>MHHHHHHSNKKSLSVIFVKPPFQLKKKFQKDPFYEI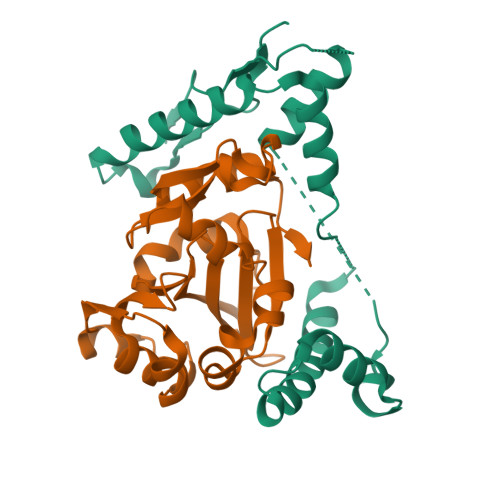EMRKQLQMQQDGINNMTIFEWLKNRENFKKYGRNPKSKKIQEDFRDRYRNAKIDEYLLLYEDMDIKAIEAMVDSELEGLAALANPAQIAGGYVDVVTQMGNKRINSSIGSQWGSIEKGRSLNIENELLKLITDPPPITEEEQKKIKMNVNLVENLEIVK[2x];>[2x]MFEKFLERSGNSIKLEEFSEDYIRQYNNLVSEKLISFWRIAGIGIYCNGLFRTIIPNDYQYIIEECYPMYDYETVTPFMITVFGDIFAYVKNHVIGDYVVFINIRYGTFKILSENIDILLNIVIFNKSCLENWFLLNEYNTIKEVKAMPKIDECYGYVPALVAGGKDCIDNIQIVKIAPYIDTVIQLMGDLKRIR> MGSSHHHHHHHHGASENLYFQGASMTFSNADAQKIAVQKDVDEVVAAAQRFLHGSGNATSDEAKVDLQKKASNLVQTIRGPIPAALSSMEDIVKVASLRTLFEAGVFHAMPKGGASMTASEISAQTGLDKGILIRLMRAVTPLGPFHEVGEEEYAHTPFSEAYLTADIAGCFPVMSNFIFGPVLQICDFLRQNNWKDAITTRNNPFTLAHNCPGETMFEHLYKNSKNVAPVTKAEAADVD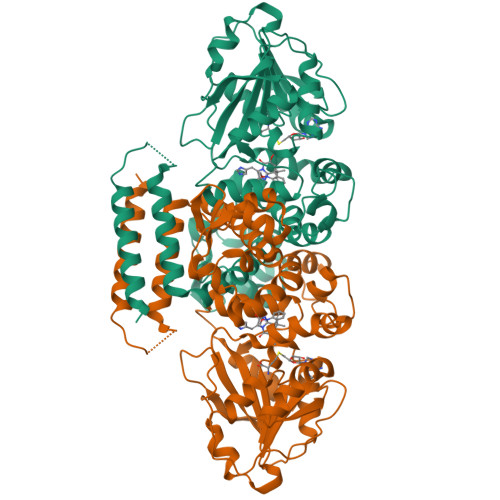QIAMDLYPWEERLSDAKGSNATLVDIAGSHGNGTRAIMALAPKLNGCRFIVQDLEPVIGEHSQALRAEGIEPQVYDFLKQEQPVHGASIYYFRRVFHDWPDLPEGKKILDNTRAAMSREHSRILIHDIIVPEIGATMSHAWQDLSLMAIGGMERTEKDFARLLDIAGLALVKVWRKPGDMMGIIEARLK Copper-containing nitrite reductases (CuNiRs) are found in all three kingdoms of life and play a major role in the denitrification branch of the global nitro­gen cycle where nitrate is used in place of di­oxy­gen as an electron acceptor in respiratory energy metabolism. The catalytic type-2 copper center (T2Cu) is located at the interface of the adjacent monomers and is ‘hard-wired’ to the electron-donating type-1 copper center (T1Cu) via neighboring residues that form a Cys–His electron-transfer (ET) bridge. The two active-site residues, AspCAT and HisCAT around the T2Cu, are involved in substrate binding and catalysis with both residues starting in the deprotonated state prior to substrate-binding events. The hexameric structure observed for the N-terminal cupredoxin-tethered three-domain CuNiR from two strains of Hyphomicrobium denitrificans suggests that it is likely to offer an advantage for these organisms.

In both of these HdNiRs, the T1CuN in the N-terminal tethered cupredoxin domain is placed at a distance of ∼24 Å from the catalytic core T1Cu, which may be considered too far away for an effective electron transfer. A close examination of the structural differences between the two HdNiRs was made with particular emphasis on the non-conserved amino-acid residues between the two enzymes. These residues are predominantly located on the surface of the N-terminal tethered cupredoxin domain, which is exposed to solvent [Fig. S3(c)], though some are also in the inter- and/or intra monomer interface. Despite the fact that HdNiR from two different strains of bacteria crystallize in different space groups, neither structure shows electron density for the N-terminal peptide, reflecting the intrinsic high flexibility of the region. Interestingly, comparison among these shows different structural arrangements around the T2Cu including the positioning of His27 in the flexible N-terminal peptide. For the ligand water (W1)-bound structure [Fig. 3(a)], the N-terminal His27 assumes an outward open conformation, where a single water molecule is positioned near the His27.

>MAADAPAASQQSKPSESDKSESSMSSHAPVVFTLRTGIAEGRMVYIGVGGDIDRQVNPKLVVHEGETVQINLINGEGAQHDAVIDQYAARSAIVSGKNASSTFSFIASKVGQFDYYCSLPGHRQAGMQGVLQVVPGNRAEMPSTAADITRDPADLPGPIGARQAKTVRIDLETVELKGQLDDKTTYTYWTFNGKVPGPFLRVRVGDTVELHLKNAKDSLMIHSVDFHGATGPGGAAAYTQTDPGAETVVTFKALVPGIFVYHCATPSVPNHITNGMYGLLLVEPEGGLPQVDREFYVMQGEIYTVKPFGTSGEQEMDYEKLISEKPEYFLFNGSVGALTRTHPLYANVGETVRIFFGVGGPNFTSSFHVIGEIFDHVYALGSVTSPPLTGVQTVSVPPGGATIVDFKLDRGGRYVLVDHALSRLDHGLVGFLNVDGPKNDAIMHEGPPKQENLYFQ[3x]HP activity is regulated by its first and rate-limiting enzyme glutamine fructose-6-phosphate amidotransferase (GFAT, EC 2.6.1.16). GFAT is a modular enzyme composed of a glutaminase domain responsible for hydrolysis of l-Gln into l-glutamate (l-Glu) and an isomerase/transferase domain that catalyzes the isomerization of Frc6P to glucose-6-phosphate (Glc6P) as well as the transfer of ammonia to Glc6P to build glucosamine-6-phosphate (GlcN6P). The relative orientation of the two domains with their respective active sites is relevant for catalysis and affected by substrate binding. GFAT-1 activity is modulated by UDP-GlcNAc feedback inhibition and via phosphorylation by protein kinase A (PKA).

We aimed to mechanistically understand the effect of Ser205 phosphorylation and generated a GFAT-1 S205D mutant to mimic the phosphorylation. To analyze the molecular consequence of the S205D substitution in human GFAT-1, we solved the crystal structure at 2.22 Å resolution. In the S205D crystal structure, we did not observe major structural differences compared to wild type GFAT-1. Notably, the PKA target residue Ser205 is located in a loop of the glutaminase domain pointing towards the glutaminase active site and the interdomain cleft between the glutaminase and isomerase domains. Ser205 is thus optimally positioned to influence domain interactions upon phosphorylation. Overall GlcN6P synthesis was decreased ~5-fold in the phospho-mimic mutant (kcat/Km: 4.4 mM−1 sec−1) compared to wild type GFAT-1 (kcat/Km: 21.3 mM−1 sec−1). Strikingly, the dose-dependent inhibition by UDP-GlcNAc was completely abolished in the S205D variant. Compared to wild type GFAT-1, the S205D mutant showed strongly reduced thermal stability of the glutaminase domain, as indicated by the specific reduction of the lower melting point. Instead, its reduced thermal stability is likely caused by altered interactions between the glutaminase and isomerase domains. We propose that Ser205 phosphorylation suppresses UDP-GlcNAc inhibition by stabilizing the glutaminase and isomerase domains in a catalytically productive orientation.

>CGIFAYLNYHVPRTRREILETLIKGLQRLEYRGYDSAGVGFDGGNDKDWEANACKIQLIKKKGKVKALDEEVHKQQDMDLDIEFDVHLGIAHTRWATHGEPSPVNSHPQRSDKNNEFIVIHNGIITNYKDLKKFLESKGYDFESETDTETIAKLVKYMYDNRESQDTSFTTLVERVIQQLEGAFALVFKSVHFPGQAVGTRRGDPLLIGVRSEHKLSTDHIPILYRTGKDKKGSCNLSRVDSTTCLFPVEEKAVEYYFASDASAVIEHTNRVIFLEDDDVAAVVDGRLSIHRIKRTAGHHHHHHDHPGRAVQTLQMELQQIMKGNFSSFMQKEIFEQPESVVNTMRGRVNFDDYTVNLGGLKDHIKEIQRCRRLILIACGTSYHAGVATRQVLEELTELPVMVELASDFLDRNTPVFRDDVCFFLSQSGETADTLMGLRYCKERGALTVGITNTVGSSISRETDCGVHINAGPEIGVASTKAYTSQFVSLVMFALMMCDDRISMQERRKEIMLGLKRLPDLIKEVLSMDDEIQKLATELYHQKSVLIMGRGYHYATCLEGALKIKEITYMHSEGILAGELKHGPLALVDKLMPVIMIIMRDHTYAKCQNALQQVVARQGRPVVICDKEDTETIKNTKRTIKVPHSVDCLQGILSVIPLQLLAFHLAVLRGYDVDFPRNLAKSVTVE[2x]> GSAAAPLSPAWMPAYACQRPTPLTHHNTGLSEALEILAEAAGFEGSEGRLLTFCRAASVLKALPSPVTTLSQLQGLPHFGEHSSRVVQELLEHGVCEEVERVRRSERYQTMKL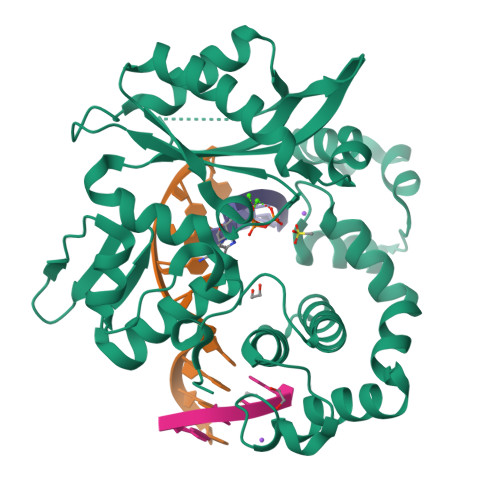FTQIFGVGVKTADRWYREGLRTLDDLREQPQKLTQQQKAGLQHHQDLSTPVLRSDVDALQQVVEEAVGQALPGATVTLTGGFRRGKLQGHDVDFLITHPKEGQEAGLLPRVMCRLQDQGLILYHQHQHSCCESPTRLAQQSHMDAFERSFCIFRLPQPGSWKAVRVDLVVAPVSQFPFALLGWTGSKLFQRELRRFSRKEKGLWLNSHGLFDPEQKTFFQAASEEDIFRHLGLEYLPPEQRNA>[2x]ATNGKLFPWAQIRLPTAVVPLRYELSLHPNLTSMTFRGSVTISVQALQVTWNIILHSTGHNISRVTFMSAVSSQEKQAEILEYAYHGQIAIVAPEALLAGHNYTLKIEYSANISSSYYGFYGFSYTDESNEKKYFAATQFEPLAARSAFPCFDEPAFKATFIIKIIRDEQYTALSNMPKKSSVVLDDGLVQDEFSESVKMSTYLVAFIVGEMKNLSQDVNGTLVSI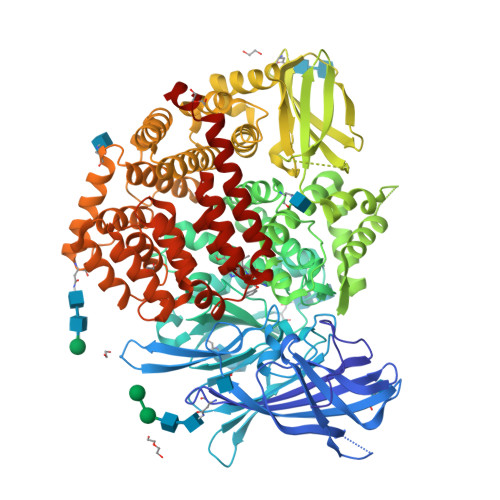YAVPEKIGQVHYALETTVKLLEFFQNYFEIQYPLKKLDLVAIPDFEAGAMENWGLLTFREETLLYDSNTSSMADRKLVTKIIAHELAHQWFGNLVTMKWWNDLWLNEGFATFMEYFSLEKIFKELSSYEDFLDARFKTMKKDSLNSSHPISSSVQSSEQIEEMFDSLSYFKGSSLLLMLKTYLSEDVFQHAVVLYLHNHSYASIQSDDLWDSFNEVTNQTLDVKRMMKTWTLQKGFPLVTVQKKGKELFIQQERFFLNMKPEIQPSDTSYLWHIPLSYVTEGRNYSKYQSVSLLDKKSGVINLTEEVLWVKVNINMNGYYIVHYADDDWEALIHQLKINPYVLSDKDRANLINNIFELAGLGKVPLKRAFDLINYLGNENHTAPITEALFQTDLIYNLLEKLGYMDLASRLVTRVFKLLQNQIQQQTWTDEGTPSMRELRSALLEFACTHNLGNCSTTAMKLFDDWMASNGTQSLPTDVMTTVFKVGAKTDKGWSFLLGKYISIGSEAEKNKILEALASSEDVRKLYWLMKSSLNGDNFRTQKLSFIIRTVGRHFPGHLLAWDFVKENWNKLVQKFPLGSYTIQNIVAGSTYLFSTKTHLSEVQAFFENQSEATFRLRCVQEALEVIQLNIQWMEKNLKSLTWWL>VDFKLSPSQLEARRHAQAFANTVLTKASAEYSTQKDQLSRFQATRPFYREAVRHGLIKAQVPIPLGGTMESLVHESIILEELFAVEPATSITIVATALGLMPVILCDSPSLQEKFLKPFISGEGEPLASLMHSEPNGTANWLQKGGPGLQTTARKVGNEWVISGEKLWPSNSGGWDYKGADLACVVCRVSDDPSKPQDPNVDPATQIAVLLVTRETIANNKKDAYQILGEPELAGHITTSGPHTRFTEFHVPHENLLCTPGLKAQGLVETAFAMSAALVG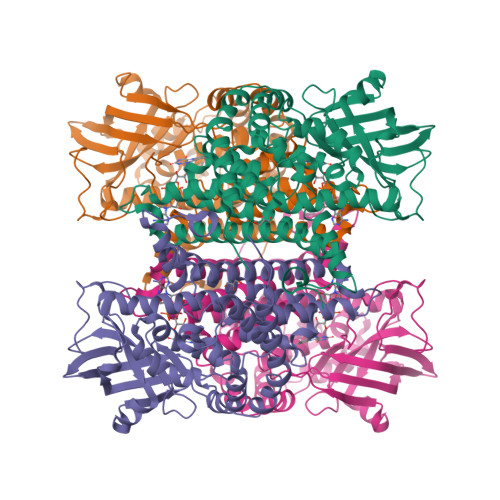AMAIGTARAAFEEALVFAKSDTRGGSKHIIEHQSVADKLIDCKIRLETSRLLVWKAVTTLEDEALEWKVKLEMAMQTKIYTTDVAVECVIDAMKAVGMKSYAKDMSFPRLLNEVMCYPLFNGGNIGLRRRQMQRVMALEDYEPWAATYGSSKVDKSRL[4x]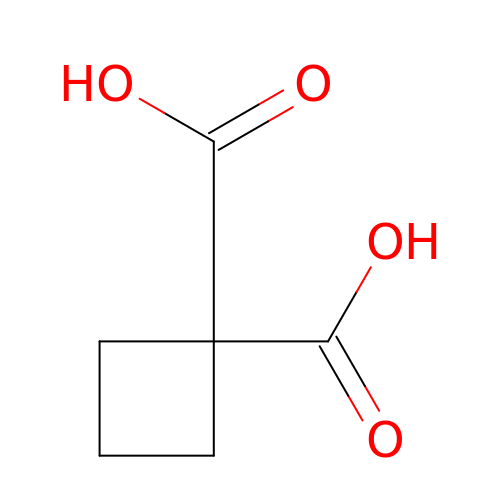cyclobutane-1,1-dicarboxylic acid | C6 H8 O4 | CCQPAEQGAVNNIA-UHFFFAOYSA-N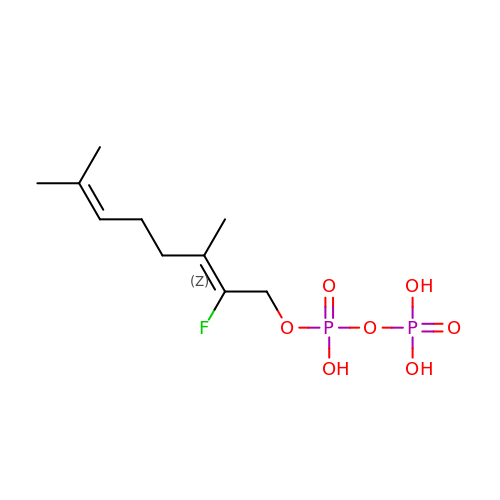(2Z)-2-fluoro-3,7-dimethylocta-2,6-dien-1-yl trihydrogen diphosphate | C10 H19 F O7 P2 | BYJNSLXDWGDGAC-KTKRTIGZSA-N> MGSSHHHHHHSQDPMEIDELTALGGLLANIGKPVQRAGLY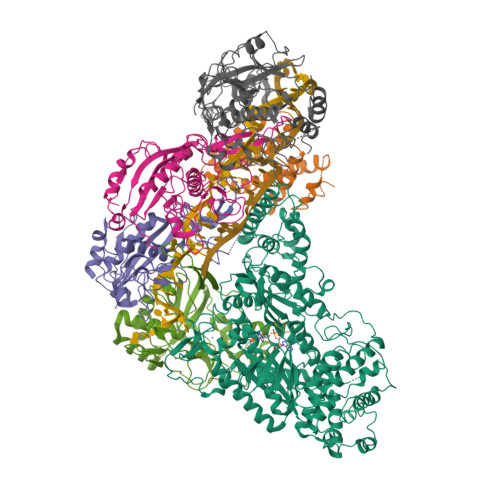SGDHSTQGARFLRDLAENTGRAEYELLSLFSEFHHKGHMKNDELMIRRIKELSPERFGLTMEDVLNALWIVYEADNLASGEREEGQPQASRPLYSVFNPGKAYPWAELDFEKELPVPGDVFSIRSQDYRELVKRLWEELSKAKLRSDRLLPVLEKYLTFVSSVTSEGNIISLYDHMRMTSAIALAMLRAGCTAEDVRSGRCRKEKRFLLIEGDFSGIQDFIYRVSGKGTLKYLRARSAYLELIGWDVVLEILSRLGLTRANVVFNAGGHFMIIAQNTPDAVKELEEIRAKAVEWLYREFESDLYLAIEWEPVSGREFGREGGKNLFAEARKRLKHKLTVRKLKRFGEIKGLFEHGHTERLAECPVCGRELPEGKLEPSASDPETKVCPTCNRLVSLGGNLPKLLGFGRTAKNDAGVLVEGPFSGFVPYLQGGRPVGEQILVKNTLNPGEIPESAQFVPYFVADYFKKDPKGGVATFEELSMASTGTRRLGVMKGDVDRLGEFFSSMDSPSKLATASRFMDYFFKGYIGAIIEGKFGYIIGDVPSLRDWPEEPDIVVVYAGGDDFFIVGAWDQIFELAFRVRRAFNAYTGGKLTLSVGLGYFDERTPIYRMADVVSERLDTAKDEGRNRVFVVGRSRPLDGKHKLSYEWNHYEELWRTYAPRIYAGNGRLKGKLESKKGLLWKLLEIRELYVRDPNDVRWAYLTAYLLGRHGLSDLFPELVGIDTKAVERKEPQPVYWVDGVLKIVLMAVRR;> SMAYHQKHGGYGRGGYGRQDRPQVDASRLFGESPDVVGIKKMLEGKGKQWEAIQPYFDNVVREAKNFLEWSPNKRLANAVTVAAYLTSQGLKTNQVRKILDMARTTELKVKRGEGDIKDDLVKMRYLLAYTVGKATGQSKYSLDAFHRILDPMLEVLMGSPKKENFEKFYDFLQAVVAYHKFFGGGD;>[2x]SMDRRFYGKIVIKGKIKAVTGLHIGSQRDISEIGGIDNPVIKDPHTGLPYIPGSSLKGRLRSLFEILVNSRLGEWREKYPSLANYSPGSCRPDNQENCGKFFNRKINRGWIHVCPDYETALACPVCRLFGASGKESNFPSRIIVRDAFLTKEWEEKWRAGEAITEAKIEVGIDRVTSQANPRTNERVVAGAEFEFEIIYNVENTTHWRDDIKNLLTAMALLEDSYLGGSGSRGYGKVKFIFDSFEFRPLDYYRTGKDEDIVSIDAREKSVSDILSGFDSLFSEVEGKLEAG;> MPKFIAVKLIPKGPFRDIPRADTLFGAIGNAISAIHGQSAVEELVDAFVGGARISSAFPYSGDTYYLPKPLSVEPALEGILTGLDEEERYTTAKRLRKAKYLDLKNFELALRLRPFTIPEEIPYARVDVPRVVLDRVTQDSSIYFWEEIRFREKSGVYFLYSGPREVFDGYIAPAMRFLGDTGIGGKSTWGAGLFEVEFHEMKIDAPGSEYSVTLSNALPTKTPVLWRLLRKGGWSFGRRKPRMTFIAEGSIVKNDPGGMERLELGLSHEVYVYGLTFPLGVELPEGLE>HRKNGGKPDHVESDISYAVARQLAVNLGLTGYQSLPPGIAKNLARGKPLPPGIAKKTVPASMLGQLPYYPGYEWKIVGDNLVLIALSTAV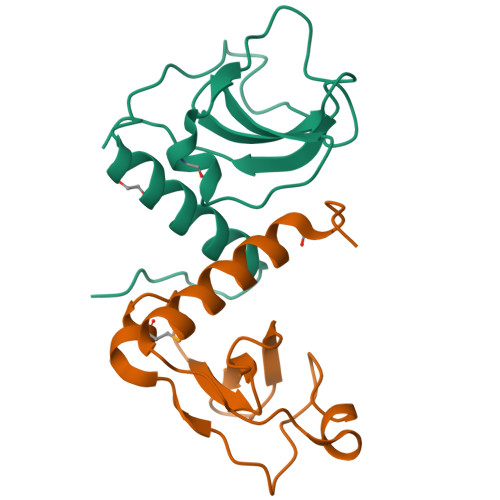VTAIINGVFDLE[2x]>MLNRVVLVGRLTKDPELRSTPNGVNVGTFTLAVNRTFTNAQGEREADFINVVVFKKQAENVKNYLSKGSLAGVDGRLQTRNYENKDGQRVFVTEVVADSVQFLEPKHHHHHH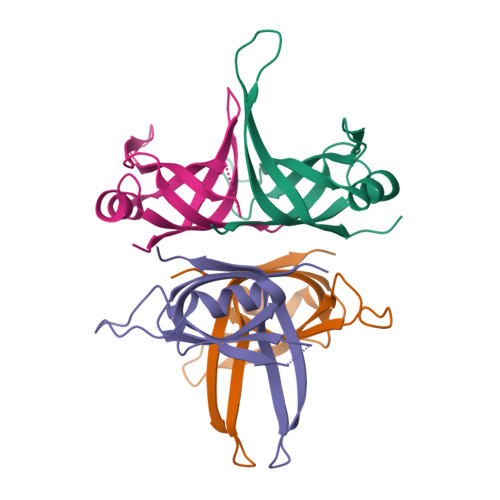[4x]> GPDSMKETPLSNCERRFLLRAIEEKKRLDGRQTYDYRNIRISFGTDYGCCIVELGKTRVLGQVSCELVSPKLNRATEGILFFNLELSQMAAPAFEPGRQSDLLVKLNRLMERCLRNSKCIDTESLCVVAGEKVWQIRVDLHLLNHDGNIIDAASIAAIVALCHFRRPDVSVQGDEVTLYTPEERDPVPLSIHHMPICVSFAFFQQGTYLLVDPNEREERVMDGLLVIAMNKHREICTIQSSGGIMLLKDQVLRCSKIAGVKVAEITELILKALENDQKVRKEGGKFGFAESIANQRITAFKMEKAPIDTSDVEEKAEEIIAEAEPPSEVVSTPVLWTPGTAQIGEGVENSWGDLEDSEKEDDEGGGDQAIILDGIKMDTGVEVSDIGSQDAPIILSDSEEEEMIILEPDKNPKKIRTQTTSAKQEKAPSKKPVKRRKKKRAAN;> GPDSMAGLELLSDQGYRVDGRRAGELRKIQARMGVFAQADGSAYIEQGNTKALAVVYGPHEIRGSRARALPDRALVNCQYSSATFSTGERKRRPHGDRKSCEMGLQLRQTFEAAILTQLHPRSQIDIYVQVLQADGGTYAACVNAATLAVLDAGIPMRDFVCACSAGFVDGTALADLSHVEEAAGGPQLALALLPASGQIALLEMDARLHEDHLERVLEAAAQAARDVHTLLDRVVRQHVREASILLGD;> RSMAAGFKTVEPLEYYRRFLKENCRPDGRELGEFRTTTVNIGSISTADGSALVKLGNTTVICGVKAEFAAPSTDAPDKGYVVPNVDLPPLCSSRFRSGPPGEEAQVASQFIADVIENSQIIQKEDLCISPGKLVWVLYCDLICLDYDGNILDACTFALLAALKNVQLPEVTINEETALAEVNLKKKSYLNIRTHPVATSFAVFDDTLLIVDPTGEEEHLATGTLTIVMDEEGKLCCLHKPGGSGLTGAKLQDCMSRAVTRHKEVKKLMDEVIKSMKPK;> RSMEEETHTDAKIRAENGTGSSPRGPGCSLRHFACEQNLLSRPDGSASFLQGDTSVLAGVYGPAEVKVSKEIFNKATLEVILRPKIGLPGVAEKSRERLIRNTCEAVVLGTLHPRTSITVVLQVVSDAGSLLACCLNAACMALVDAGVPMRALFCGVACALDSDGTLVLDPTSKQEKEARAVLTFALDSVERKLLMSSTKGLYSDTELQQCLAAAQAASQHVFRFYRESLQRRYSKS;> GPDSMASVTLSEAEKVYIVHGVQEDLRVDGRGCEDYRCVEVETDVVSNTSGSARVKLGHTDILVGVKAEMGTPKLEKPNEGYLEFFVDCSASATPEFEGRGGDDLGTEIANTLYRIFNNKSSVDLKTLCISPREHCWVLYVDVLLLECGGNLFDAISIAVKAALFNTRIPRVRVLEDEEGSKDIELSDDPYDCIRLSVENVPCIVTLCKIGYRHVVDATLQEEACSLASLLVSVTSKGVVTCMRKVGKGSLDPESIFEMMETGKRVGKVLHASLQSVVHKEESLGPKRQKVGFLG;> GPDSMPGDHRRIRGPEESQPPQLYAADEEEAPGTRDPTRLRPVYARAGLLSQAKGSAYLEAGGTKVLCAVSGPRQAEGGERGGGPAGAGGEAPAALRGRLLCDFRRAPFAGRRRRAPPGGCEERELALALQEALEPAVRLGRYPRAQLEVSALLLEDGGSALAAALTAAALALADAGVEMYDLVVGCGLSLAPGPAPTWLLDPTRLEEERAAAGLTVALMPVLNQVAGLLGSGEGGLTESWAEAVRLGLEGCQRLYPVLQQSLVRAARRRGAAAQP;> GSGSGSGSGSGSGSGSGSMAEPASVAAESLAGSRARAARTVLGQVVLPGEELLLPEQEDAEGPGGAVERPLSLNARACSRVRVVCGPGLRRCGDRLLVTKCGRLRHKEPGSGSGGGVYWVDSQQKRYVPVKGDHVIGIVTAKSGDIFKVDVGGSEPASLSYLSFEGATKRNRPNVQVGDLIYGQFVVANKDMEPEMVCIDSCGRANGMGVIGQDGLLFKVTLGLIRKLLAPDCEIIQEVGKLYPLEIVFGMNGRIWVKAKTIQQTLILANILEACEHMTSDQRKQIFSRLAES;> GPDSMAMEMRLPVARKPLSERLGRDTKKHLVVPGDTITTDTGFMRGHGTYMGEEKLIASVAGSVERVNKLICVKALKTRYIGEVGDIVVGRITEVQQKRWKVETNSRLDSVLLLSSMNLPGGELRRRSAEDELAMRGFLQEGDLISAEVQAVFSDGAVSLHTRSLKYGKLGQGVLVQVSPSLVKRQKTHFHDLPCGASVILGNNGFIWIYPTPEHKEEEAGGFIANLEPVSLADREVISRLRNCIISLVTQRMMLYDTSILYCYEASLPHQIKDILKPEIMEEIVMETRQRLLEQEG;> GPDSMAPPVRYCIPGERLCNLEEGSPGSGTYTRHGYIFSSLAGCLMKSSENGALPVVSVVRETESQLLPDVGAIVTCKVSSINSRFAKVHILYVGSMPLKNSFRGTIRKEDVRATEKDKVEIYKSFRPGDIVLAKVISLGDAQSNYLLTTAENELGVVVAHSESGIQMVPISWCEMQCPKTHTKEFRKVARVQPEFLQT;> GPDSMLKSKTFLKKTRAGGVMKIVREHYLRDDIGCGAPGCAACGGAHEGPALEPQPQDPASSVCPQPHYLLPDTNVLLHQIDVLEDPAIRNVIVLQTVLQEVRNRSAPVYKRIRDVTNNQEKHFYTFTNEHHRETYVEQEQGENANDRNNRAIRVAAKWYNEHLKKMSADNQLQVIFITNDRRNKEKAIEEGIPAFTCEEYVKSLTANPELIDRLACLSEEGNEIESGKIIFSEHLPLSKLQQGIKSGTYLQGTFRASRENYLEATVWIHGDNEENKEIILQGLKHLNRAVHEDIVAVELLPKSQWVAPSSVVLHDEGQNEEDVEKEEETERMLKTAVSEKMLKPTGRVVGIIKRNWRPYCGMLSKSDIKESRRHLFTPADKRIPRIRIETRQASTLEGRRIIVAIDGWPRNSRYPNGHFVRNLGDVGEKETETEVLLLEHDVPHQPFSQAVLSFLPKMPWSITEKDMKNREDLRHLCICSVDPPGCTDINDALHCRELENGNLEVGVHIADVSHFIRPGNALDQESARRGTTVYLCEKRIDMVPELLSSNLCSLKCDVDRLAFSCIWEMNHNAEILKTKFTKSVINSKASLTYAEAQLRIDSANMNDDITTSLRGLNKLAKILKKRRIEKGALTLSSPEVRFHMDSETHDPIDLQTKELRETNSMVEEFMLLANISVAKKIHEEFSEHALLRKHPAPPPSNYEILVKAARSRNLEIKTDTAKSLAESLDQAESPTFPYLNTLLRILATRCMMQAVYFCSGMDNDFHHYGLASPIYTHFTSPIRRYADVIVHRLLAVAIGADCTYPELTDKHKLADICKNLNFRHKMAQYAQRASVAFHTQLFFKSKGIVSEEAYILFVRKNAIVVLIPKYGLEGTVFFEEKDKPNPQLIYDDEIPSLKIEDTVFHVFDKVKVKIMLDSSNLQHQKIRMSLVEPQIPGISIPTDTSNMDLNGPKKKKMKLGK;> GPDSASMAAERKTKLSKNLLRMKFMQRGLDSETKKQLEEEEKKIISEEHWYLDLPELKEKESFIIEEQSFLLCEDLLYGRMSFRGFNPEVEKLMLQMNAKHKAEEVEDETVELDVSDEEMARRYETLVGTIGKKFARKRDHANYEEDENGDITPIKAKKMFLKPQD

The eukaryotic RNA exosome is a conserved and versatile ribonuclease complex involved in many RNA quality-control and turnover pathways in both nuclear and cytoplasmic compartments. Proteomic studies of human exosome complexes recently showed that the 9-subunit barrel associates with two distinct yRrp44 orthologues, hDIS3 and hDIS3L, to form nucleoplasmic and cytoplasmic hEXO-10 complexes, respectively. Here, we report a mechanistic comparison of the human and yeast nuclear exosomes with the aim to understand the extent of their evolutionary conservation and to identify species-specific features.

We engineered a catalytically inactive mutant of human hDIS3 (hDIS3cat Asp146Asn, Asp487Asn) analogous to the previously characterized yRrp44 mutant (yRrp44cat Asp171Asn, Asp551Asn [Bonneau et al., 2009]). Upon 2D classification and initial 3D classification, we observed two distinct particle populations that were then subjected separately to another round of 3D classification. From the larger particle population we obtained the structure of human hEXO-10cat-hMPP6 at 3.80 Å resolution and from a smaller one we obtained the structure of hEXO-14cat at 6.25 Å resolution (Figure 2—figure supplements 1–3). The human hEXO-10cat-hMPP6 cryo-EM structure revealed unambiguous density for the hEXO-9 barrel and for the hDIS3 ribonuclease. In the cryo-EM structure, hCSL4 is only partially ordered. Similarly to the yeast exosome structure, the corresponding CR3 motif of hDIS3 forms a long β-hairpin wedged between hRRP41-hRRP42. However, the CR3 motif of hDIS3 is twenty-residue shorter and lacks a yRrp41-interacting loop (corresponding to yRrp44 residues 60–67). In hDIS3, the CSD lobe is separated from the S1 lobe by a large funnel-like cleft, reminiscent of OB fold arrangement present in RNase II and DIS3L2. In the cryo-EM structure, the overall position of the hDIS3 exoribonuclease region on hEXO-9 does not resemble the closed conformation with which yeast yRrp44 binds RNAs entering from the long channel path but rather the open conformation with which yeast Rrp44 binds RNA in the direct access path. When inspecting the reconstructed 3D volume for un-modeled density features, we could observe a tube of density corresponding to a long single-stranded RNA bound in the channel path of hEXO-10. The long RNA channel path in the human exosome is thus formed by the combination of an open conformation of hDIS3 and an apical entry to the exoribonuclease active site.N-[(2S)-2-(3,5-dichlorophenyl)-2-(ethylamino)acetyl]-3-methyl-L-valyl-N-[3-(methylsulfonyl)propyl]glycinamide 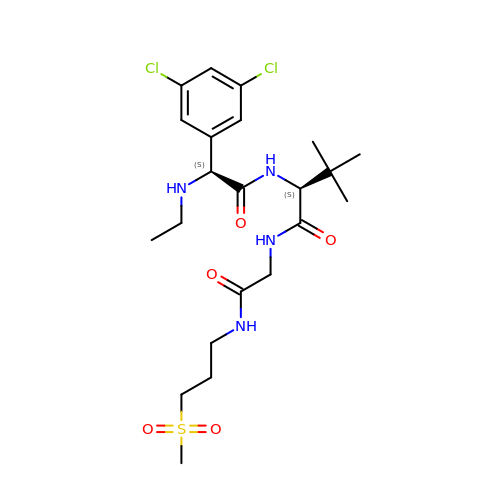| C22 H34 Cl2 N4 O5 S | ZSBXAULTZFUUMY-RBUKOAKNSA-N> GAMKSRYTTEF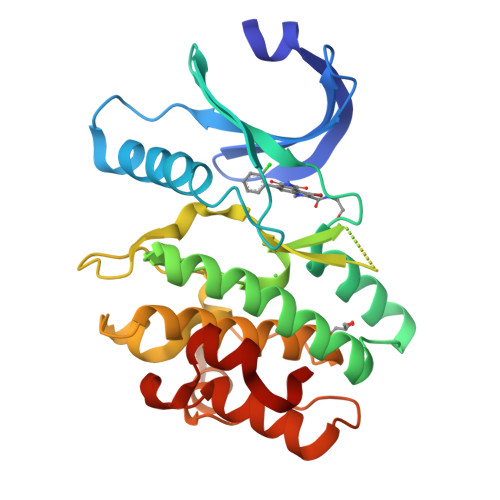HELEKIGSGEFGSVFKCVKRLDGCIYAIKRSKKPLAGSVDEQNALREVYAHAVLGQHSHVVRYFSAWAEDDHMLIQNEYCNGGSLADAISENYRIMSYFKEAELKDLLLQVGRGLRYIHSMSLVHMDIKPSNIFISRTSIPNAASEEGDEDDWASNKVMFKIGDLGHVTRISSPQVEEGDSRFLANEVLQENYTHLPKADIFALALTVVCAAGAEPLPRNGDQWHEIRQGRLPRIPQVLSQEFTELLKVMIHPDPERRPSAMALVKHSVLLSASRK>SYQPTSLTVASYNLRNANGSDSARGDGWGQRYPVIAQMVQYHDFDIFGTQECFLHQLKDMKEALPGYDYIGVGRDDGKDKGEHSAIF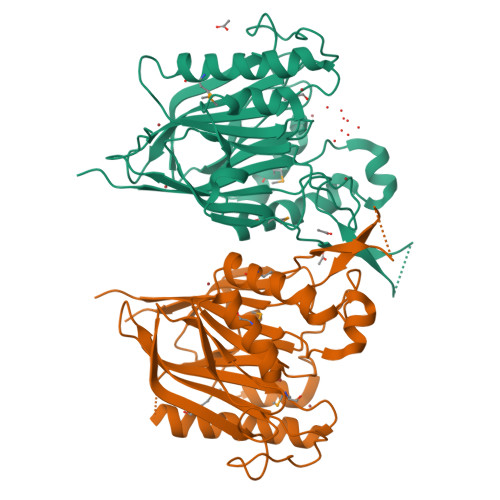YRTDKFDIVEKGDFWLSETPDVPSKGWDAVLPRICSWGHFKCKDTGFEFLFFNLHMDHIGKKARVESAFLVQEKMKELGRGKNLPAILTGDFNVDQTHQSYDAFVSKGVLCDSYEKCDYRYALNGTFNNFDPNSFTESRIDHIFVSPSFHVKRYGVLTDTYRSVRENSKKEDVRDCPEEITIKAYEARTPSDHFPVKVELVFDLEHHHHHH[4x]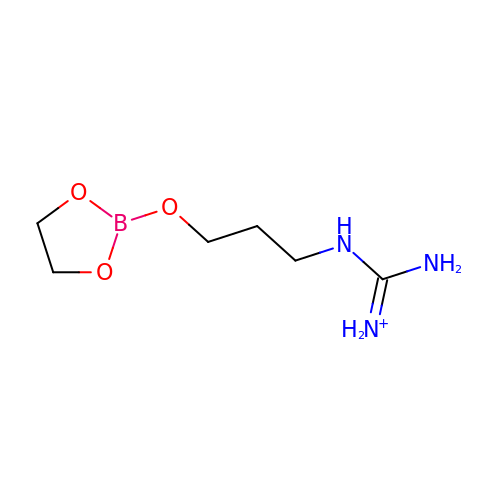[3-(1,3,2-DIOXABOROLAN-2-YLOXY)PROPYL]GUANIDINE | C6 H15 B N3 O3 | QHANCKHXGBJANE-UHFFFAOYSA-O> MSLQPKRIHYMVKVGDTLSGIFAQLGVPYSILQKILSVDLDHLQLDMIQPGEELELMMDDMGQLSRLIYHMSIVEKAIYTRENDGSFSYDFQEISGEWREILFSGEINGSFSVSARRVGLTSSQVANITQVMKDKIDFSRSLRAGDRFDILVKQQ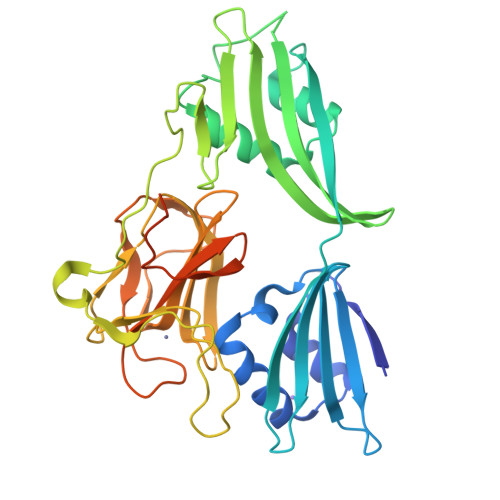YLGEHNTGNSEIKAISFKLAKGDVSAFLAEDGRFYDRAGNSLERAFNRYPVDKAYRQITSGFNPKRKHPVTGRVVPHNGTDFATPIGAPVYSTGDGKVIVVRKHPYAGNYLVIEHNSVYKTRYLHLDKILVKKGQLVKRGQKIALAGATGRLTGPHLHFEVLVRNRPVDAMKADLPIAKSLSSNQKTSFLARVSEFDHEGHHHHHH URIC ACID | C5 H4 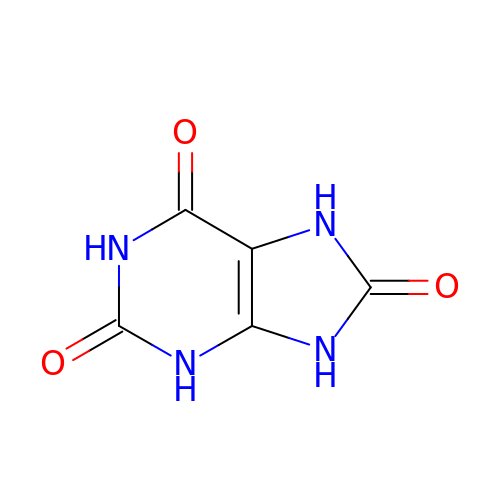N4 O3 | LEHOTFFKMJEONL-UHFFFAOYSA-N> TENILRKSDEEIQKEITARVKALESMLIEQGILTTSMIDRMAEIYENEVGPHLGAKVVVKAWTDPEFKKRLLADGTEACKELGIGGLQGEDMMWVENTDEVHHVVVCTLCSCYPWPVLGLPPNWFKEPQYRSRVVREPRQLLKEEFGFEVPPSKEIKVWDSSSEMRFVVLPQRPAGTDGWS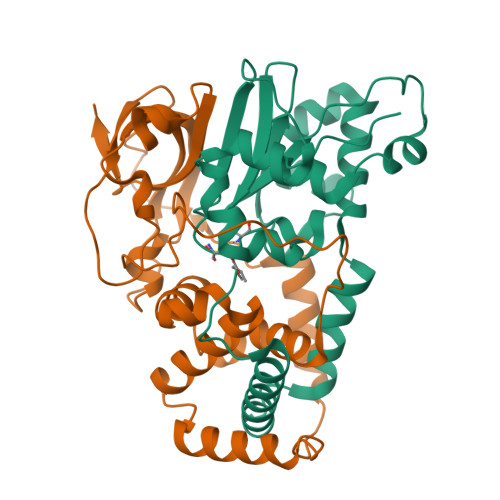EEELATLVTRESMIGVEPAKAV;> MNGVYDVGGTDGLGPINRPADEPVFRAEWEKVAFAMFPATFRAGFMGLDEFRFGIEQMNPAEYLESPYYWHWIRTYIHHGVRTGKIDLEELERRTQYYRENPDAPLPEHEQKPELIEFVNQAVYGGLPASREVDRPPKFKEGDVVRFSTASPKGHARRARYVRGKTGTVVKHHGAYIYPDTAGNGLGECPEHLYTVRFTAQELWGPEGDPNSSVYYDCWEPYIELV> SNATDTAEQVIASFRILASDKPYILAEELRRELPPDQAQYCIKRMPAYSGPGSVPGALDYAAFSSALYGESDL;> SMMATITCTRFTEEYQLFEELGKGAFSVVRRCVKVLAGQEYAAKIINTKKLSARDHQKLEREARICRLLKHPNIVRLHDSISEEGHHYLIFDLVTGGELFEDIVAREYYSEADASHCIQQILEAVLHCHQMGVVHRDLKPENLLLA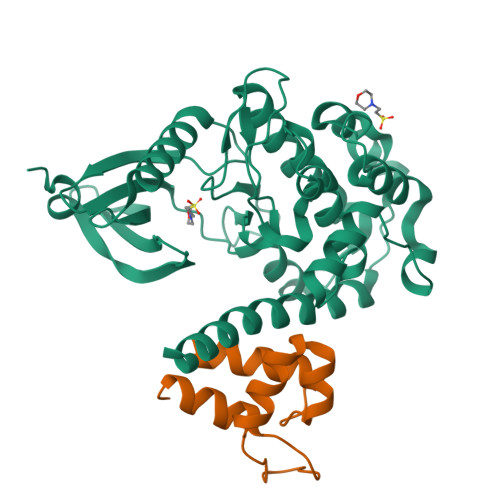SKLKGAAVKLADFGLAIEVEGEQQAWFGFAGTPGYLSPEVLRKDPYGKPVDLWACGVILYILLVGYPPFWDEDQHRLYQQIKAGAYDFPSPEWDTVTPEAKDLINKMLTINPSKRITAAEALKHPWISHRSTVASCMHRQETVDCLKKFNARRKLKGAILAAMLATRNFSG>MVVIGEKFPEVEVKTTHGVIKLPDYFAEQGKWFVLFSHPADFTPVSTTEFYAMQKRVDQFRELGVEPIGLSVDQVFSHIKWMEWIKENLGEEITFPVIADDRGELADKLGMIPSGATITARAVFIVDDKGIIRAIVYYPAEVGRDWDEILRLVKALKVSDEKGVALPHKWPNNELIGDKAIVPPASTVDEVKQREEAKAKGEIESYDWWF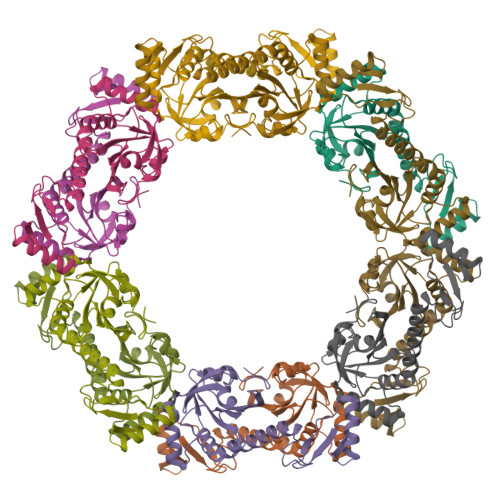SYKKLE[2x]> SNAAGCSSDKATGGSEATGPDGVKQGPGVTDKTIKLGIATDLTGVYAPLGKSITQAQQLYYEEVNQRGGVCGR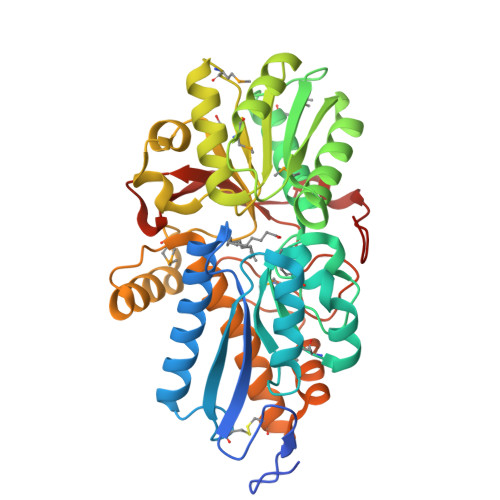TIEAVVRDHGYDPQKAVSIYTELNNNVLAIPHFLGSPMVSAVKQRIESDKMFTIPSAWTTALLGSKYIQVTGTTYDVDMINGVQWLMDKKLIKKGDKLGHVYFEGDYGGSALRGTKYAAEQLGLEVFELPIKPTDRDMKSQVAALAKEKVDAILLSAGPQQAASLAGIARSQGMKQPILGSNSAYSPQLLATPAKPALVEGFFIATAGAPMSADLPAIKKLAEAYSKKYPKDPLDSGVVNGYGGASIVVSALEKACANKDLTREGLINAHRSEANADDGLGTPMNFTYFDKPATRKTYIIKPDEKATGGAVIVEQAFESELAKNYQVPVGTF> AASLAPGSSRVELFKRKNSTVPFEESNGTIRERVVHSFRIPTIVNVDGVMVAIADARYETSFDNSFIETAVKYSVDDGATWNTQIAIKNSRASSVSRVVDPTVIVKGNKLYILVGSFNKTRNYWTQHRDGSDWEPLLVVGEVTKSAANGKTTATISWGKPVSLKPLFPAEFDGILTKEFVGGVGAAIVASNGNLVYPVQIADMGGRVFTKIMYSEDDGNTWKFAEGRSKFGCSEPAVLEWEGKLIINNRVDYNRRLVYESSDMGKTWVEALGTLSHVWTNSPTSNQPDCQSSFVAVTIEGKRVMLFTHPLNLKGRWMRDRLHLWMTDNQRIFDVGQISIGDENSGYSSVLY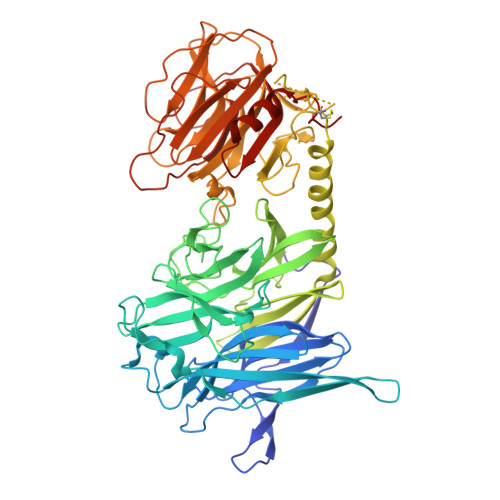KDDKLYSLHEINTNDVYSLVFVRLIGELQLMKSVVRTWKEEDNHLASICTPVVPATPPSKGACGAAVPTAGLVGFLSHSANGSVWEDVYRCVDANVANAERVPNGLKFNGVGGGAVWPVARQGQTRRYQFANYRFTLVATVTIDELPKGTSPLLGAGLEGPGDAKLLGLSYDKNRQWRPLYGAAPASPTGSWELHKKYHVVLTMADRQGSVYVDGQPLAGSGNTVVRGATLPDISHFYIGGPRSKGAPTDSRVTVTNVVLYNRRLNSSEIRTLFLSQDMIGTDGGAGTAA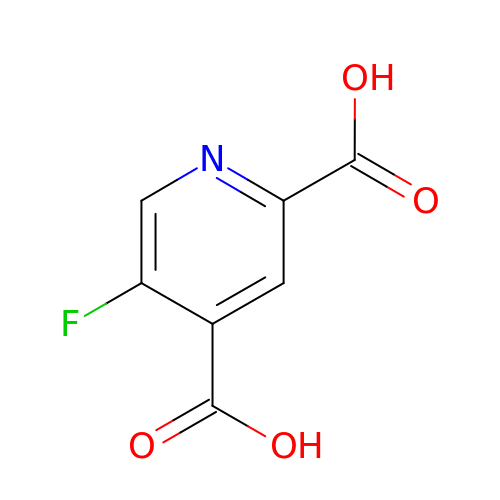5-fluoranylpyridine-2,4-dicarboxylic acid | C7 H4 F N O4 | YMTWJDCPCBQOIJ-UHFFFAOYSA-N> GSSLRQEPSGQGLGVALKSTPGILSGKLPESVSDVRFSSPQGQGESRTLTDSAGPRQITLRQFENGVTELQLSRPPLTSLVLSGGGAKGAAYPGAMLALEEKGMLDGIRSMSGSSAGGITAALLASGMSPAAFKTLSDKMDLISLLDSSNKKLKLFQHISSEIGASLKKGLGNKIGGFSELLLNVLPRIDSRAEPLERLLRDETRKAVLGQIATHPEVARQPTVAAIASRLQSGSGVTFGDLDRLSAYIPQIKTLNITGTAMFEGRPQLVVFNASHTPDLEVAQAAHISGSFPGVFQKVSLSDQPYQAGVEWTEFQDGGVMINVPVPEMIDKNFDSGPLRRNDNLILEFEGEAGEVAPDRGTRGGALKGWVVGVPALQAREMLQLEGLEELREQTVVVPLKSERGDFSGMLGGTLNFTMPDEIKAHLQERLQERVGEHLEKRLQASERHTFASLDEALLALDDSMLTSVAQQNPEITDGAVAFRQKARDAFTELTVAIVSANGLAGRLKLDEAMRSALQRLDALADTPERLAWLAAELNHADNVDHQQLLDAMRGQTVQSPV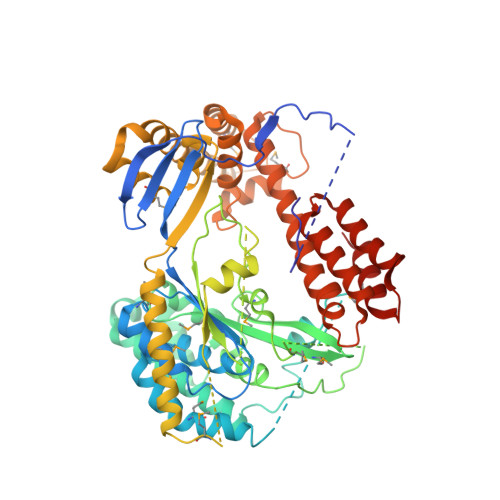LAAALAEAQRRKVAVIAENIRKEVIFPSLYRPGQPDSNVALLRRAEEQLRHATSPAEINQALNDIVDNYSARGFLRFGKPLSSTTVEMAKAWRNKEFT>GMKSSQPFIYEAHAARV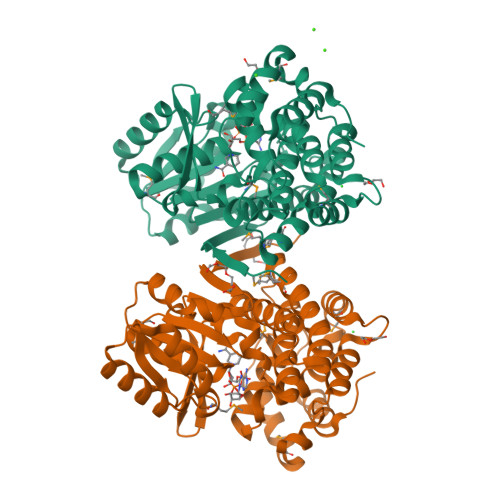VFGAGSSSQVAAEVERLGAKRALVLCTPNQQAEAERIADLLGPLSAGVYAGAVMHVPIESARDATARAREAGADCAVAVGGGSTTGLGKAIALETGMPIVAIPTTYAGSEVTPVYGLTEAGTKRTGRDPRVLPRTVIYDPALTVGLPRGLSVTSALNAIAHAAEGLYARDANPVMSLMAEEGIRALAAGIPAVFNDPADLDARSQCLYGAWLCGTVLGGVGMALHHKLCHTLGGSFNLPHAETHTIVLPHALAYNAAAVPEAMARIRRATGAGEQSAAATLFDLAQRHGAPVALRDIGMREEDLDRAADIALASPYWNPRPIEREPIRALLQAAYEGVRPD[4x]> MRRLFLLLAWQPSFAKHLSELEPVPQRAPVEKRRRQHI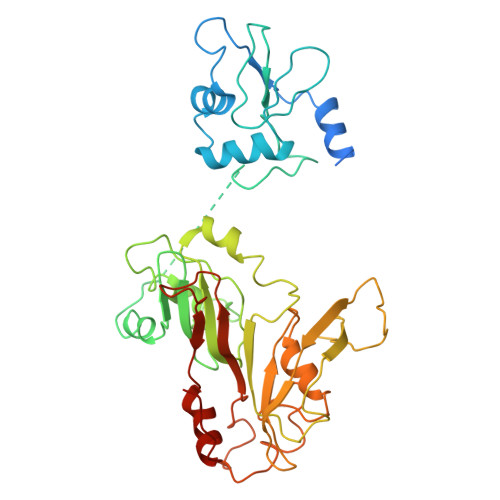PLSLQAREELSRKSNELQYHVVTQDWFGQRVDDFVTQHHPEWDYETVKRLVQQGHIYRYRKNGKKRYTRLTDRLEFDELVVVPTASFWERQLAPPSGVELQSSSTSQQQERRQKFHLSAKTREMAQEMVLFKNEHVIVINKPSGVPIMPTHDPLAMNITDLLPAWRYTNTQTPVICHNLDTETSGCVVLARSANTHRMLGRMFVKRVVPNSVYWGFAVGKPPVNFGRIRMHFEVQKGQGGDVIVARPTPTADSKVGIAEFVVNASALEFGSFISFYPLTTRRHQERIMAAHALRAPLLGDAKYGGESAFPHSLSLFWDPARKDVPLHLHHRKIQLPYKNGAGEFVCVTAPLPPHMEKTFKRLGWPVDADDPLIPG>[4x]SNADDLREPEERH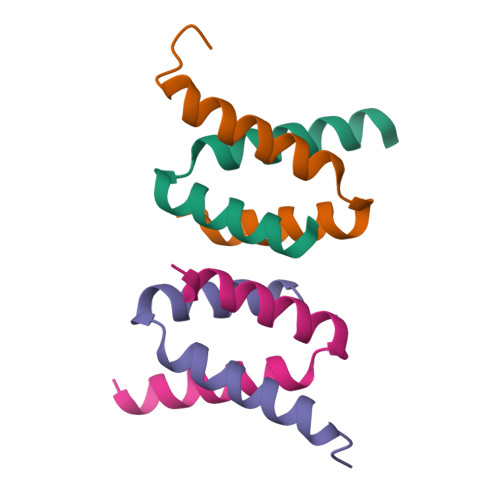LDDAFFRGYKNLEPEAKAQLRKILDTFKKDF> MAELACFCYPHLENDSYKFIPFNNLAIKAMLTAKVDKKDMDKFYDSIIYGIAPPPQFKKRYNTNDNSRGMNFETIMFTKVAMLICEALNSLKVTQANVSNVLSRVVSIRHLENLVIRKENPQDIL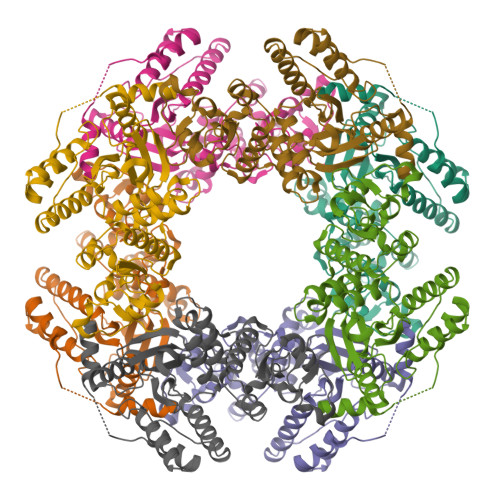FHSKDLLLKSTLIAIGQSKEIETTITAEGGEIVFQNAAFTMWKLTYLEHQLMPILDQNFIEYKVTLNEDKPISDVHVKELVAELRWQYNKFAVITHGKGAYRIVKYSSVANHADRVYATFKSNVKTGVNNDFNLLDQRIIWQNWYAFTSSMKQGNTLDVCKRLLFQKMKPEKNPFKGLSTDRKMDEVSQVGV> MGSSHHHHHHSSGLVPRGSALSPPRRKAFKKWTPPRSPFNLVQETLFHDPWKLLIATIFLNRTSGKMAIPVLWKFLEKYPSAEVARTADWRDVSEL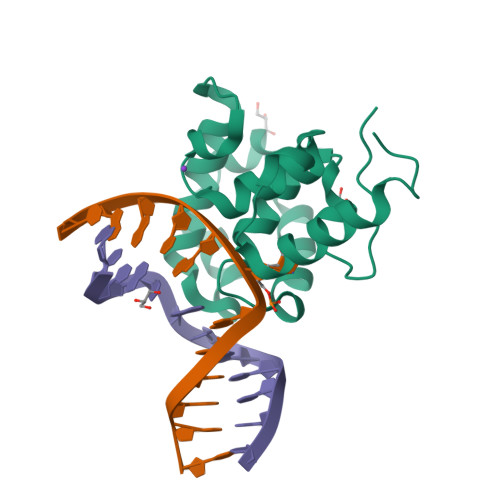LKPLGLYDLRAKTIVKFSDEYLTKQWKYPIELHGIGKYGNDSYRIFCVNEWKQVHPEDHKLNKYHDWLWENHEKLSLS> SPFSIFHPNIQAAKDCNQVRDFITKEVDSDVNTAEWGTFVAVSTPGRKDRDADMASSSTPRFRVYSKYLFLTYPQCTLEPQYALDSLRTLLNKYEPLYIAAVRELHEDGSPHLHVLVQNKLRASITNPNALNLRMDT

HUH endonucleases are diverse enzymes that contain an eponymous motif consisting of a pair of conserved metal-coordinating histidine (H) separated by a bulky hydrophobic residue (U). Replication-initiating HUH endonucleases (Reps) are sequence-specific nucleases that cleave and rejoin single-stranded DNA (ssDNA) during rolling-circle replication. Replication initiator proteins (Reps) from this HUH endonuclease superfamily are found in a variety of bacterial plasmids and viral genomes, including circular Rep-encoding single-stranded DNA (CRESS-DNA) viruses that are known to infect organisms across all three domains of life (1–5). These enzymes initiate rolling-circle replication through sequence-specific processing of the viral single-stranded DNA (ssDNA) genome via cleavage and subsequent phosphotyrosine covalent linkage to the ssDNA’s newly exposed 5′ end. Following linkage, the genome’s freed 3′-OH can be used as a primer for DNA replication before its ultimate return to the active site, where it attacks the phosphotyrosine intermediate to rejoin and release the circular ssDNA genome.

The first cocrystal structures of viral Reps in complex with their specific substrates provided insight into their mechanisms of DNA recognition. Strikingly, the ssDNA conforms into a distinct U shape around a key topologically stabilizing motif in the Rep called the single-stranded DNA bridging motif (sDBM). A common feature across all structures of CRESS-DNA viral Reps in complex with their ssDNA substrates elucidated thus far is an intramolecular WC base pair between the −4T and +1A positions with respect to the cleavage site.> GPHAGIVLTKVGYYTIPSMDDLAKITNEKG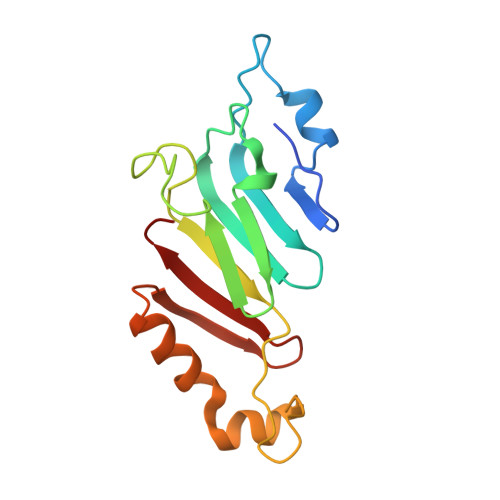ECIVSDFTIGRKGYGSIYFEGDVNLTNLNLDDIVHIRRKEVIVYVDDNQKPPVGEGLNRKAEVTLDGVWPTDKTSRCLIKSPDRLADINYEGRLEAVSRKQGAQFKEYRPETGSWVFKVSHF The largest of these factors, eIF3, is a multi-subunit complex consisting of five stoichiometric subunits in yeast (eIF3a, b, c, g and i). One of its large subunits, eIF3b, serves as a scaffold within eIF3 as it interacts with several other subunits. Here, by using X-ray crystallography we studied the structure of yeast eIF3b-RRM and showed that it corresponds to the canonical RNA recognition motif. The structure is composed of four β-strands and two α-helices which are arranged in a β-α-β-β-α-β sequential order.

Two different truncations of the N-terminal domain of yeast eIF3b were designed based on homology to the published structure of its human ortholog. Crystals of the shorter truncation (rsidues 76–161) diffracted to 2.6 Å. However, they were not easily reproducible as bunches of needles were obtained instead. Comparison of the relative orientation of the monomers between eIF3b-RRM76–170 and eIF3b-RRM76–161 showed that chain B in eIF3b-RRM76–161 has been displaced by ∼9 Å relative to the same chain in eIF3b-RRM76–170. Therefore this dimer is most probably an artifact of the crystallization and not the functional unit of the protein in the solution. This is in agreement with the gel-filtration profile of the protein showing that it eluted from the column at a volume corresponding to the size of about 10 kDa (data not shown).

>[2x]GPLGSDQYIVVNGAPVIPSAKVPVLKKALTSLFSKAGKVVNMEFPIDEATGKTKGFLFVECGSMNDAKKIIKSFHGKRLDLKHRLFLYTMK>[2x]MRLCDRDIEAWLDEGRLSINPRPPVERINGATVDVRLGNKFRTFRGHTAAFIDLSGPKDEVSAALDRVMSDEIVLDEGEAFYLHPGELALAV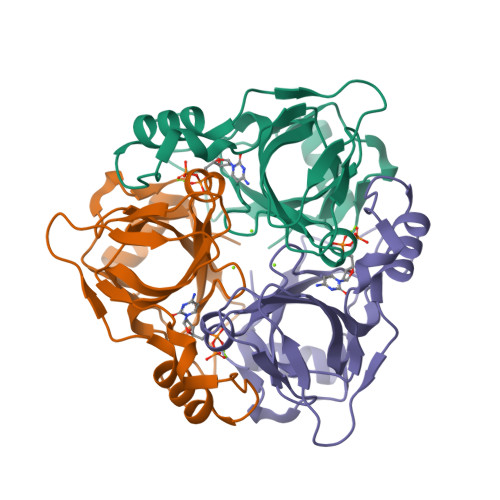TLESVTLPADLVGWLDGRSSLARLGLMVAVTAHRIDPGWSGCIVLEFYNSGKLPLALRPGMLIGALSFEPLSGPAVRPYNRREDAKYRNQQGAVASRIDKD The cap intermediate is methylated by the RNA guanine N-7 methyltransferase, utilising the methyl donor, AdoMet, to create the mature cap, m7GpppN, and byproduct, AdoHcy (S-adenosyl homocysteine). In mammals, RNA guanylyltransferase and 5′-triphosphatase (RNGTT/CE) caps the nascent transcript and RNA guanine-7 methyltransferase (RNMT) methylates the cap. Human RNMT is a 476 amino acid nuclear protein consisting of a catalytic domain (residues 121–476), with homology to other eukaryotic cap methyltransferases and an N-terminal regulatory domain (residues 1–120), that mediates recruitment to transcription initiation sites. RNMT also has an activating subunit, RAM (RNMT-activating miniprotein).

Here we report the structure of human RNMT in complex with RAM. Two complexes within an asymmetric unit were found to perfectly superpose (RMSD 0.46 Å RNMT chain A versus B; RMSD 0.22 Å RAM chain C versus D). In the RNMT–RAM crystal structure, RAM 2–45 binds to a positively charged surface groove on RNMT, distal to the active site. This groove comprises of the RNMT α-helix hinge containing helices G and H (residues 395–415) and the lobe. The interface between RNMT and RAM was analysed using the PISA server (EMBLI-EBI) revealing an average interface area of 1695 Å2. Eleven amino acids in RAM spanning R18 to W43 are involved in polar interactions with RNMT, and RAM E25, R32 and E42 establish salt bridges with RNMT K392, E397 and R450. Many residues involved in these interactions lie in the RNMT lobe (residues 416–456), which co-evolved with RAM in vertebrates. The most overt effect of RAM binding is the stabilisation and resolution of the RNMT lobe, residues 416–456. Secondary structure element attribution using the DSSP program revealed the lobe to consist of a β-sheet made of two small anti-parallel β-strands (10a and 10b), which flank the α-helix L. The RNMT–RAM crystal structure in conjunction with biochemical analyses and molecular dynamics simulations has revealed that RAM activates RNMT by stabilising the RNMT lobe and α-helix hinge, thus positioning adjacent helix A in the active site in a position favourable for substrate binding and the methylation reaction.

>SQSRIFYLRNFNNWMKSVLIGEFLEKVRQKKKRDITVLDLGCGKGGDLLKWKKGRINKLVCTDIADVSVKQCQQRYEDMKNRRDSEYIFSAEFITADSSKELLIDKFRDPQMCFDICSCQFVCHYSFESYEQADMMLRNACERLSPGGYFIGTTPNSFELIRRLEASETESFGNEIYTVKFQKKGDYPLFGCKYDFNLEGVVDVPEFLVYFPLLNEMAKKYNMKLVYKKTFLEFYEEKIKNNENKMLLKRMQALEPYPANESSKLVSEKVDDYEHAAKYMKNSQVRLPLGTLSKSEWEATSIYLVFAFEKQQ[2x];>TDTAEAVPKFEEMFASRFTENDKEYQEYLKRPPESPPIVEEWNS[2x]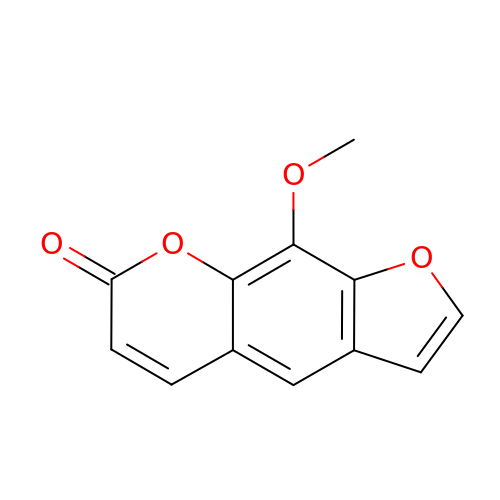METHOXSALEN | C12 H8 O4 | QXKHYNVANLEOEG-UHFFFAOYSA-N>GMHIQPGLCGLGNLGNTCFMNSALQCLSNTAPLTDYFLKDEYEAEINRDNPLGMKGEIAEAYAELIKQMWSGRDAHVAPRMFKTQVGRFAPQFSGYQQQDSQELLAFLLDGLHEDLNRVKKKPYLELKDANGRPDAVVAKEAWENHRLRND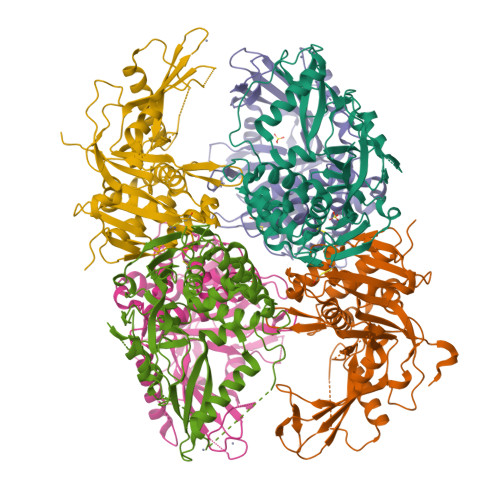SVIVDTFHGLFKSTLVCPECAKVSVTFDPFCYLTLPLPLKKDRVMEGPMLQPQKKKKTTVALRDCIELFTTMETLGEHDPWYCPNCKKHQQATKKFDLWSLPKILVVHLKRFSYNRYWRDKLDTVVEFPIRGLNMSEFVCNLSARPYVYDLIAVSNHYGAMGVGHYTAYAKNKLNGKWYYFDDSNVSLASEDQIVTKAAYVLFYQRRDDEFYKTPS[6x]> MKPPQQQHEAFPLFKGATRLPTIWGVPMIPLMAMVMGVAVIALTVSIWWWALVPPLWFIMAQITKNDDKAFRIWWLWIDTKFRNRNKGFWGASSYSPANYRK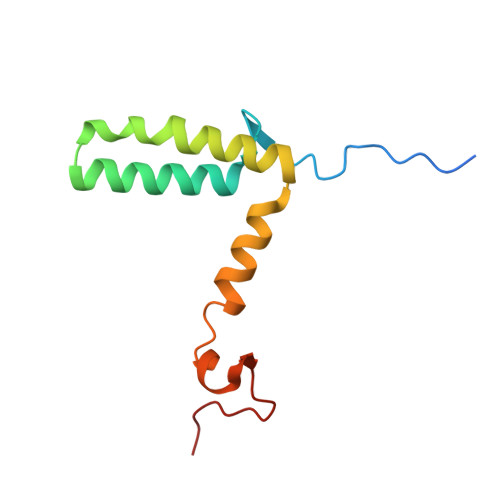RR>MVYPIRLYGDPVLRRKARPVEDFSGIKRLAEDMLETMFEAKGVGLAAPQIGLSQRLFVAVEYADEPEGEEERPLRELVRRVYVVANPVITYREGLVEGTEGCLSLPGL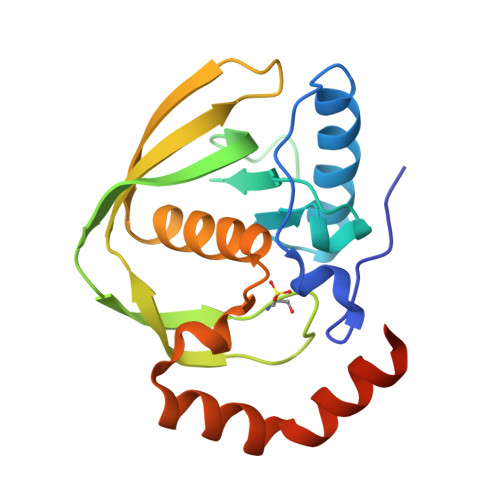YSEEVPRAERIRVEYQDEEGRGRVLELEGYMARVFQHEIDHLDGILFFERLPKPKREAFLEANRAELVRFQKEARALLKELSQG[2x]2-[[1,3-dicyclohexyl-4-oxidanyl-2,6-bis(oxidanylidene)pyrimidin-5-yl]carbonylamino]ethanoic 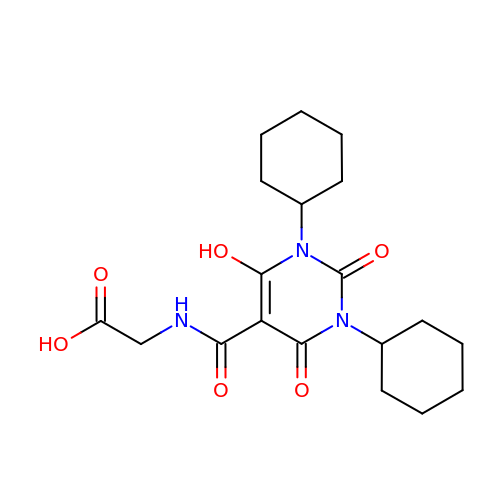acid | C19 H27 N3 O6 | NVTKJBXOBFRPLQ-UHFFFAOYSA-N> GSQKERLLDELTLEGVARYMQSERCRRVICLVGAGISTSAGIPDFRSPSTGLYDNLEKYHLPYP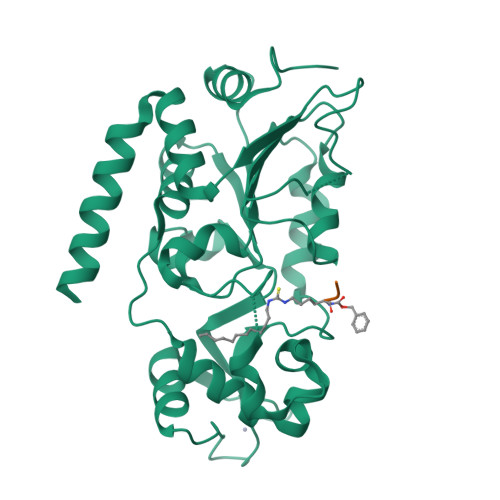EAIFEISYFKKHPEPFFALAKELYPGQFKPTICHYFMRLLKDKGLLLRCYTQNIDTLERIAGLEQEDLVEAHGTFYTSHCVSASCRHEYPLSWMKEKIFSEVTPKCEDCQSLVKPDIVFFGESLPARFFSCMQSDFLKVDLLLVMGTSLQVQPFASLISKAPLSTPRLLINKEKAGGGGMDFDSKKAYRDVAWLGECDQGCLALAELLGWKKELEDLVRREHASIDAQS> IPISMSDEGDSFLVKDSIGENKIPKNPSKVVILDLGILDTFDALKLNDKVVGVPAKNLPKYLQQFKNKPSVGGVQQVDFEAINALKPDLIIISGRQSKFYDKLKEIAPTLFVGLDNANFLSSFENNVLSVAKLYGLEKEALEKI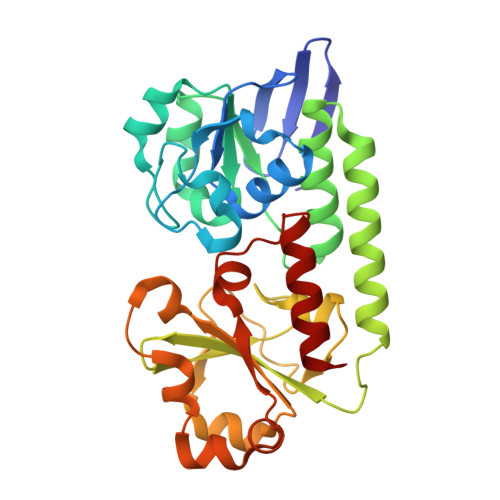SDIKNEIEKAKSIVDEDKKALIILTNSNKISAFGPQSRFGIIHDVLGINAVDENIKVGTHGKSINSEFILEKNPDYIFVVDRNVILGNKERAQGILDNALVAKTKAAQNKKIIYLDPEYWYLASGNGLESLKTMILEIKNAVK> GHMAKK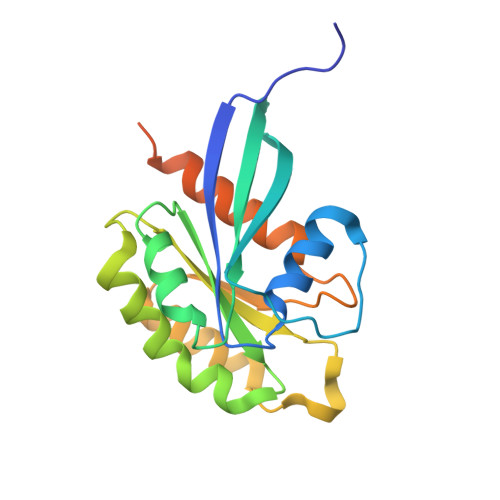TYDLLFKLLLIGDSGVGKTCVLFRFSDDAFNTTFISTIGIDFKIKTVELQGKKIKLQIWDTAGQERFHTITTSYYRGAMGIMLVYDITNGKSFENISKWLRNIDEHANEDVERMLLGNKCDMDDKRVVPKGKGEQIAREHGIRFFETSAKANINIEKAFLTLAEDILRKTPVKEPNSENVDISSGGGVTGWKSKCC> MIEPVLENVQPNSAASKAGLQAGDRIVKVDGQPLTQWVTFVMLVRDNPGKSLALEIERQGSPLSLTLIPESKPGNGKAIGFVG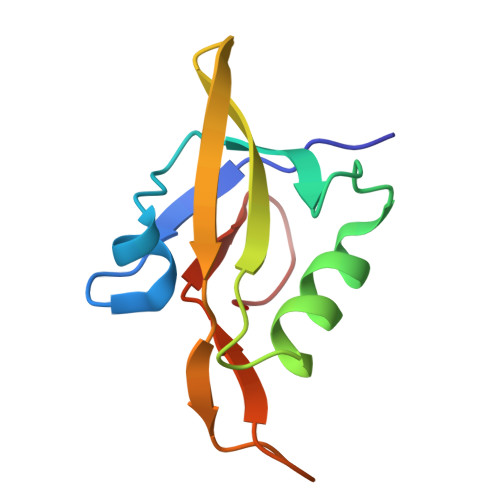IEPKGKASPV>[2x]SITPGTYNITNVAYTNRLIDLTGSNPAENTLIIGHHLNKTPSGYGNQQWTLVQLPHTTIYTMQAVNPQSYVRVRDDNLVDGAALVG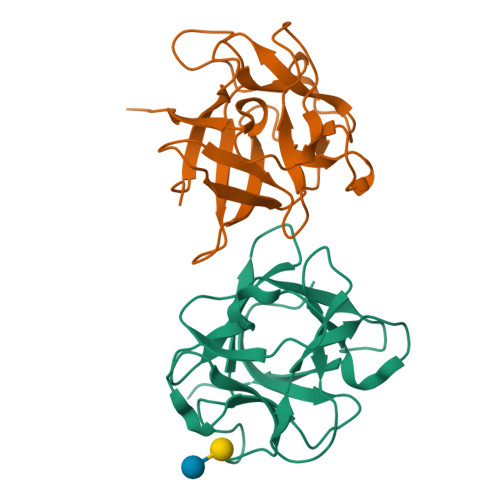SQQPTPVSIESAGNSGQFRIKIPNLGLALTLPSDANSTPIVLGEVDETSTNQLWAFESVSAV> MHHHHHHMSGGLTPDQAIDAIRGTGGAQPGCRALHAKGTLYRGTFTATRDAVMLSAAPHLDGSTVPALIRFSNGSGNPKQRDGAPGVRGMAVKFTLPDGSTTDVSAQTARLLVSSTPEGFIDLLKAMRPGLTTPLRLATHLLTHPRLLGALPLLREANRIPASYA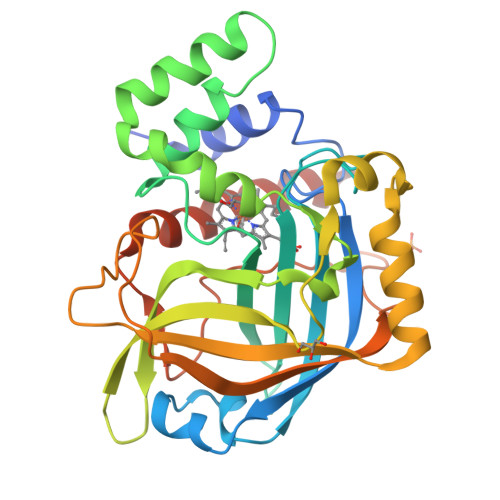TTEYHGLHAFRWIAADGSARFVRYHLVPTAAEEYLSASDARGKDPDFLTDELAARLQDGPVRFDFRVQIAGPTDSTVDPSSAWQSTQIVTVGTVTITGPDTEREHGGDIVVFDPMRVTDGIEPSDDPVLRFRTLVYSASVKLRTGVDRGAQAPPV>[4x]GPMSSVQLSRGDFHSIFTNKQRYDNPTGGVYQVYNTRKSDGANSNRENLIMISDGIYHMKALLRNQAASKFQSMELQRGDIIRVIIAEP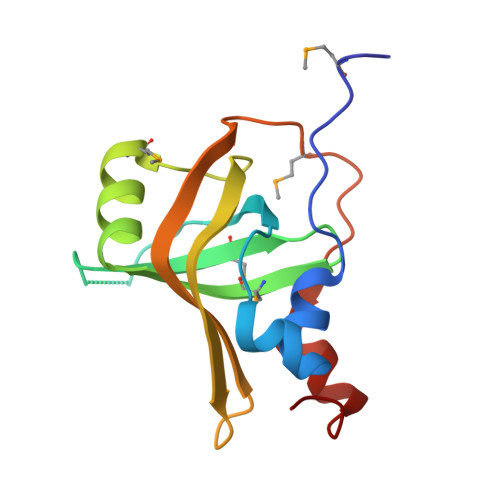AIVRERKKYVLLVDDFELVQSRADMVNQTSTFLDNYFSEHPNETL~{N}2-(1~{H}-benzimidazol-2-yl)benzene-1,2-diamine 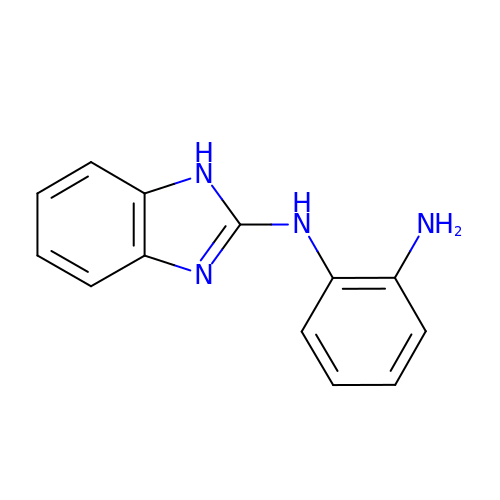| C13 H12 N4 | ZZDGNBWCSPZNRU-UHFFFAOYSA-N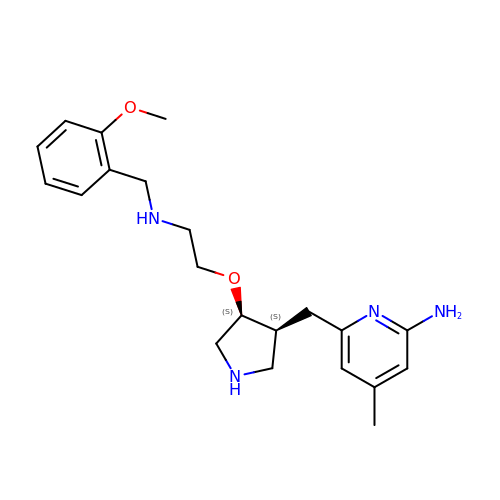6-{[(3S,4S)-4-{2-[(2-methoxybenzyl)amino]ethoxy}pyrrolidin-3-yl]methyl}-4-methylpyridin-2-amine | C21 H30 N4 O2 | CNZPKQOAIMARQF-FXAWDEMLSA-N>MQKDALNNVHITDEQVLMTPEQLKAAFPLSLQQEAQIADSRKSISDIIAGRDPRLLVVCGPCSIHDPETALEYARRFKALAAEVSDSLYLVMRVYFEKPRTTVGWKGLINDPHMDGSFDVEAGLQIARKLLLELVNMGLPLATEALDPNSPQYLGDLFSWSAIGARTTESQTHREMASGLSMPVGFKNGTDGSLATAINAMRAAAQPHRFVGINQAGQVALLQTQGNPDGHVILRGGKAPNYSPADVAQCEKEMEQAGLRPSLMVDCSHGNSNKDYRRQPAVAESVVAQIKDGNRSIIGLMIESNIHEGNQSSEQPRSEMKYGVSVTD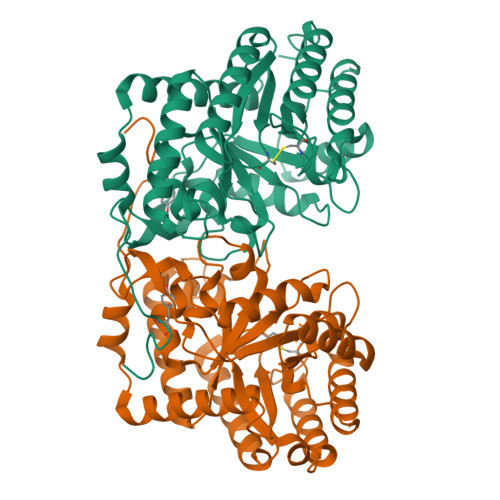ACISWEMTDALLREIHQDLNGQLTARV[4x]octopine | C9 H18 N4 O4 | 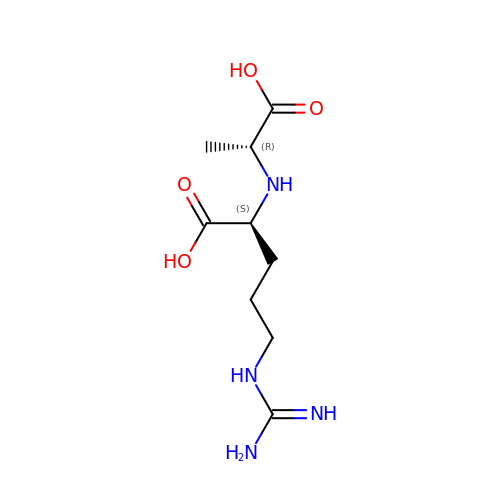IMXSCCDUAFEIOE-RITPCOANSA-N>[2x]MGHHHHHHMRVKTFVILCCALQYVAYTNANINDFDED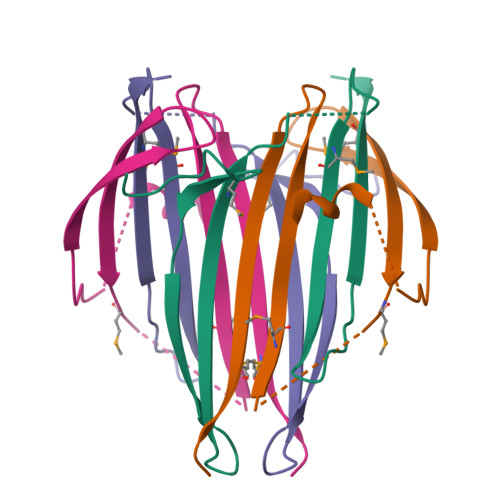YFGSDVTVQSSNTTDEIIRDASGAVIEEQITTKKMQRKNKNHGILGKNEKMIKTFVITTDSDGNESIVEEDVLMKTLSDGTVAQSYVAADAGAYSQS> ESRRESINPWILTGFADAEGSFLLRIRNNNKSSVGYSTELGFQITLHNKDKSILENIQSTWKVGVIANSGDNAVSLKVTRFEDLKVIIDHFEKYPLITQKLGDYMLFKQAFCVMENKE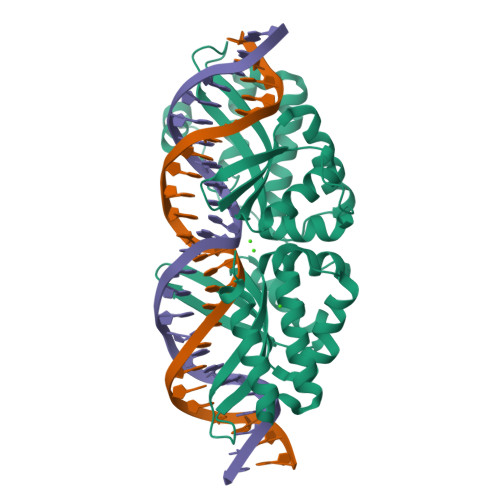HLKINGIKELVRIKAKLNWGLTDELKKAFPEIISKERSLINKNIPNFKWLAGFTSGEGCFFVNLIKSKSKLGVQVQLVFSITQHIKDKNLMNSLITYLGCGYIKEYNKSEFSWLAFVVTKFSDINDKIIPVFQENTLIGVKLEDFEDWCKVAKLIEEKKHLTESGLDEIKKIKLNMNKGRVF>[2x]MKTKFYDYQGEHLILYFAGWGTPPDAVNHLILPENHDLLICYDYQDLNLDFDLSAYRHIRLVAWSMGVWVAERVLQ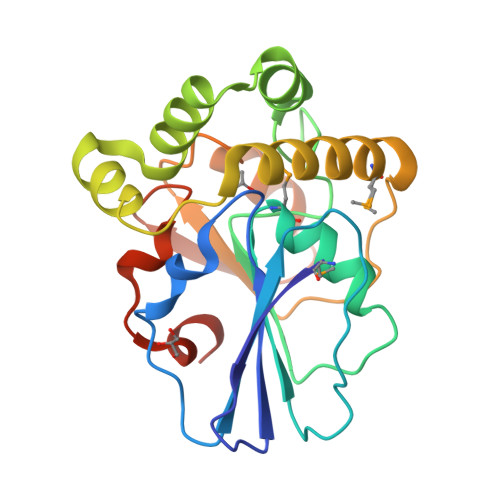GIRLKSATAVNGTGLPCDDSFGIPYAIFKGTLENLTENTRLKFERRICGDKASFERYQLFPARPFDEIHQELTALFAMIQQDKRIDLIHWANAWVSSRDKIFTPANQHQYWALRCAVQEIEGEHYVFSRFTHWSALWDHLEHHHHHH> MRLELPVIPLRNTVILPHTTTPVDVGRAKSKRAVEEAMGADRLIFLVAQRDPEVDDPAPDDLYTWGVQAVVKQAMRLPDGTLQVMVEARARAQVTDYIPGPYLRARGEVFSEIFPIDEAVVRVLVEELKEAFEKYVANHKSLRLDRYQLEAVKGTSDPAMLADTIAYHATWTVAEKQEILELTDLEARLKKVLGLLSRDLERFELDKRVAQRVKEQMDTNQREYYLREQMKAIQKELGGEDGLSDLEALRKKIEEVGMPEAVKTKALKELDRLERMQQGSPEATVARTYLDWLTEVPWSKADPEVLDINHTRQVLDEDHYGLKDVKERILEYLAVRQLTQGLDVRNKAPILVLVGPPGVGKTSLGRSIARSMNRKFHRISLGGVRDEAEIRGHRRTYIGAMPGKLIHAMKQVGVINPVILLDEIDKMSSDWRGDPASAMLEVLDPEQNNTFTDHYLDVPYDLSKVFFITTANTLQTIPRPLLDRMEVIEIPGYTNMEKQAIARQYLWPKQVRESGMEGRIEVTDAAILRVISEYTREAGVRGLERELGKIARKGAKFWLEGAWEGLRTIDASDIPTYLGIPRYRPDKAETEPQVGTAQGLAWTPVGGTLLTIEVAAVPGSGKLSLTGQLGEVMKESAQAALTYLRAHTQDYGLPEDFYNKVDL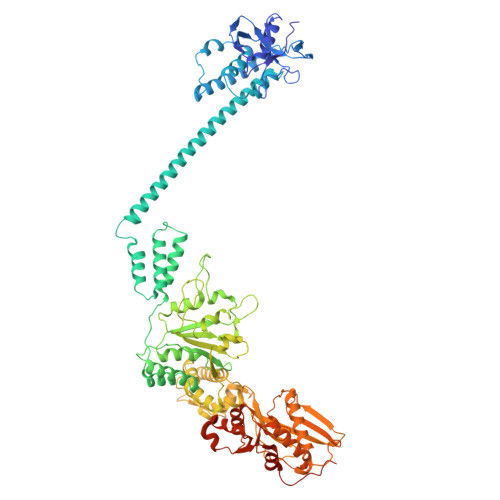HVHVPDGATPKDGPSAGITMATAIASALSRRPARMDIAMTGEVSLRGKVMPIGGVKEKLLAAHQAGIHKIVLPKDNEAQLEELPKEVLEGLEIKLVEDVGEVLEYLLLPEPTMPPVVQPSDNRQQPGAGAKLAAALEHHHHHH> GPVRLPGLAAMRQGTRLFTPEQGEDLREALRRRRGSFQTTCEVTSETTFAAARRLREKASALAALNFASAKNPGGGFLGGAQAQEEDLCRGSGLYFSLTSPQAEPYYAVNRQSHS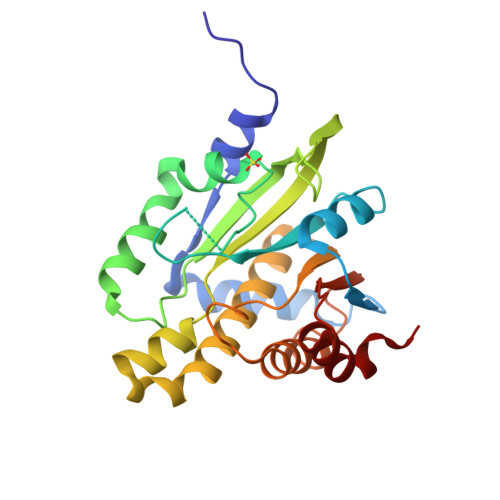ALYTDHLIYSPQVPIFRDDAGQLLPAPVPVNIITAPAPNAGAVAQSRPEQLPQVLPTLRERARRVLGVAAWMEQTHLVLGAWGCGVFRNDPAGVARTFRELLEGEAQGAFEHVTFAVLDNHPQHPTLGAFRRELESLCLP>FN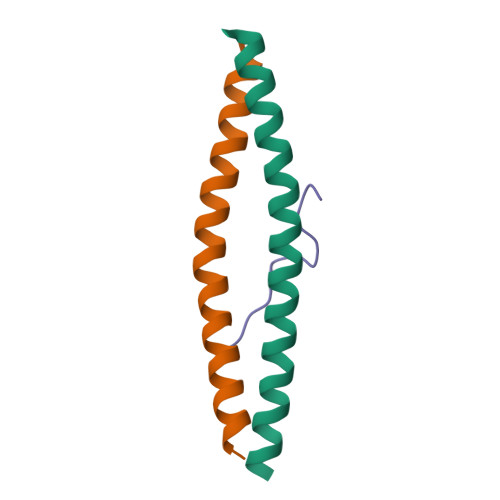SSINNIHEMEIQLKDALEKNQQWLVYDQQREVYVKGLLAKIFELEKKTETAAHSLP[2x];> QAQGPPYPTYPGY Methylenetetrahydrofolate dehydrogenase/cyclohydrolase 2 (MTHFD2) is a bifunctional metabolic enzyme found in mitochondria, exhibiting both dehydrogenase and cyclohydrolase catalytic activities. In one-carbon metabolism, MTHFD2 converts 5, 10-methylene tetrahydrofolate (5,10-CH2-THF) to 10-formyl tetrahydrofolate (10-CHO-THF) in mitochondria, thereby regulating the production of NADH, purines, and pyrimidines. An isozyme, methylenetetrahydrofolate dehydrogenase, cyclohydrolase and formyltetrahydrofolate synthetase 1 (MTHFD1), performs similar catalytic reactions to MTHFD2, albeit localized in the cytoplasm rather than the mitochondrion. The key distinction between these two proteins lie in their expression profiles: MTHFD1 is typically expressed in normal cells while MTHFD2 is abundantly expressed in immortal, embryonic, and cancer cells, but absent in adult normal cells.

Bioisosteric replacement of γ-carboxylic acid of glutamic acid with 1H-tetrazole to give 16a significantly increased the potency against MTHFD1 (IC50 = 120 nM) and MTHFD2 (IC50 = 22 nM). The structure of MTHFD2/16a revealed the headgroup, 2,5,6-triamino-3H-pyrimidin-4-one ring of 16a, establishes a hydrogen bond network with key amino acid residues, including Val131, Leu133, and Asp155. The urea moiety of 16a formed hydrogen bonds with the side chain of Lys88 and Gln132. In the middle region of 16a, the phenyl ring formed robust π–π interactions with Tyr84, and hydrophobic interactions with neighboring amino acids such as Tyr84, Ile276, Thr316, and Val317. The amide moiety adjacent to the phenyl ring was hydrogen bonded with Asn87 and participated in hydrophobic interactions with Gly313. Furthermore, the carboxylic acid moiety of 16a not only formed a hydrogen bond with the main chain of Gly310 but also established a well-organized hydrogen bond network with Gly311, Val312, and Gly313 mediated by a water molecule. Moreover, the 1H-tetrazole moiety formed hydrogen bonds with the side chain of Ser83. Superimposition of the structures of MTHFD2/16a with MTHFD2/LY374571 revealed that the 1H-tetrazole moiety in 16a exhibits an enhanced tendency for forming hydrogen bonds, either directly or through water bridging, with the side chain of Arg278 and Ser83. Moreover, the larger size of 1H-tetrazole moiety was found to form more extensive van der Waals contacts with neighboring residues such as Ile276, Leu289, and Pro309, as compared to its γ-carboxylic acid counterpart. The collective impact of these interactions contributes to the increased potency of 16a and 16g against MTHFD2.

>[2x]GSHMEAVVISGRKLAQQIKQEVRQEVEEWVASGNKRPHLSVILVGENPASHSYVLNKTRAAAVVGINSETIMKPASISEEELLNLINKLNNDDNVDGLLVQLPLPEHIDERRICNAVSPDKDVDGFHVINVGRMCLDQYSMLPATPWGVWEIIKRTGIPTLGKNVVVAGRSKNVGMPIAMLLHTDGAHERPGGDATVTISHRYTPKEQLKKHTILADIVISAAGIPNLITADMIKEGAAVIDVGINRVHDPVTAKPKLVGDVDFEGVRQKAGYITPVPGGVGPMTVAMLMKNTIIAAKKVLRLEEREVLKSKELGVATN>GPLGSMEDAKNIKKGPAPFYPLEDGTAGEQLHKAMKRYALVPGTIAFTDAHIEVNITYAEYFEMSVRLAEAMKRYGLNTNHRIVVSSENSLQFFMPVLGALFIGVAVAPANDCYNERELLNSMNISQPTVVFVSKKGLQKILNVQKKLPIIQKIIIMDSKTDYQGFQSMYTFVT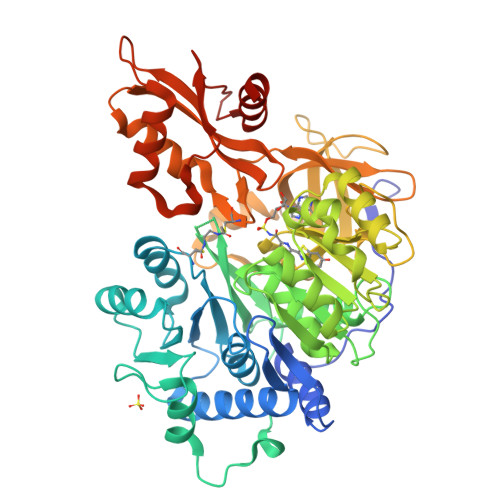SHLPPGFNEYDFVPESFDRDKTIALIMNSSGSTGLPKGVALPHRALAVRFSHARDPIFGNQIAPDTAILSVVPFHHGFGMFTTLGYLISGFRVVLMYRFEEELFLRSLQDYKIQSALLVPTLFSFLAKSTLIDKYDLSNLHEIASGGAPLSKEVGEAVAKRFHLPGIRQGYGLTETTSAILITPKGDDKPGAVGKVVPFFEAKVVDLDTGKTLGVNQRGELSVRGPMIMSGYVNNPEATNALIDKDGWLHSGDIAYWDEDEHFFIVDRLKSLIKYKGCQVAPAELESILLQHPNIFDAGVAGLPDDDAGELPAAVVVLEHGKTMTEKEIVDYVASQVTTAKKLRGGVVFVDEVPKGLTGKLDARKIREILIKAKKGGKSKL[2x]>GSMPKPINVRVTTMDAELEFAIQPNTTGKQLFDQVVKTVGLREVWFFGLQYVDSKGYSTWLKLNKKVTQQDVKKENPLQFKFRAKFFPEDVSEELIQEITQRLFFLQVKEAILNDEIYCPPETAVLLASYAVQAKYGDYNKEIHKPGYLANDRLLPQRVLEQHKLTKEQWEERIQNWHEEHRGMLREDSMMEYLKIAQDLEMYGVNYFEIKNKKGTELWLGVDALGLNIYEHDDKLTPKIGFPWSEIRNISFNDKKFVIKPIDKKAPDFVFYAPRLRINKRILALCMGNHELYMRRRKPDTIEVQQMKAQARVDSSGRIV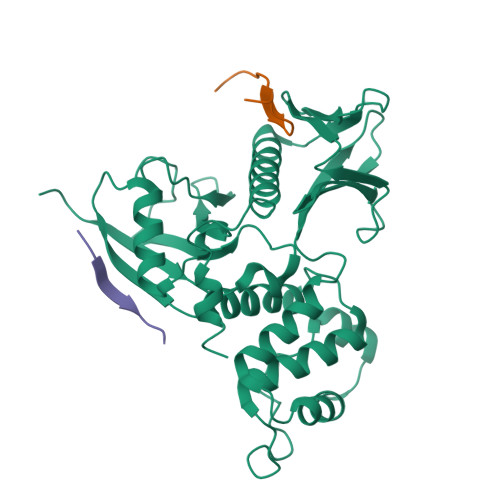TD[2x];>RLSRKTHMYPVRNYSPTE[3x]>[3x]SRCTHLENRDFVTGTQGTTRVTLVLELGGCVTITAEGKPSMDVWLDAIYQENPAKTREYCLHAKLSDTKVAARCPTMGPATLTEEHQGGTVCKRDQSDRGWGNHCGLFGKGSIVACVKAACEAKKKATGHVYDANKIVYTVKVEPHTGDYVAANETHSGRKTASFTVSSEKTILTMGEYGDVSLLCRVASGVDLAQTVILELDKTVEHLPTAWQVHRDWFNDLALPWKHEGAQNWN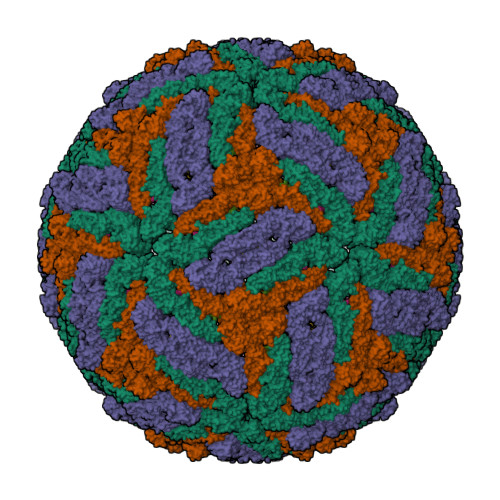NAERLVEFGAPHAVKMDVYNLGDQTGVLLKALAGVPVAHIEGTKYHLKSGHVTCEVGLEKLKMKGLTYTMCDKTKFTWKRAPTDSGHDTVVMEVTFSGTKPCRIPVRAVAHGSPDVNVAMLITPNPTIENNGGGFIEMQLPPGDNIIYVGELSHQWFQKGSSIGRVFQKTKKGIERLTVIGEHAWDFGSAGGFMTSIGRAMHTVLGGAFNTLLGGVGFLPKILLGVAMAWLGLNMRNPTLSMGFLLSGGLVLAMTLGVGA;>SVLIPSHAQGELTGRGHKWLEGDSLRTHLTRVEGWVWKNKLLALAMVTVVWLTLESVVTRVAVLVVLLCLAPVYA[3x]N-{[(2S,5S)-1-benzyl-5-(2-{[(2S,3S)-1-(tert-butylamino)-3-methyl-1-oxopentan-2-yl]amino}-2-oxoethyl)-3,6-dioxopiperazin-2-yl]methyl}-L-alpha-asparagine 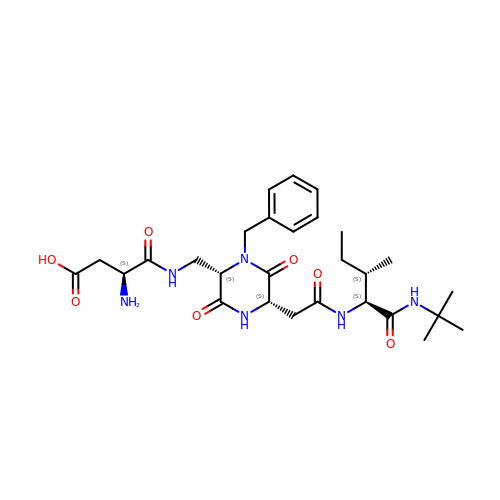| C28 H42 N6 O7 | QOSIRQNYWJNZFB-WGLQCKHLSA-N> MTIKVGINGFGRIGRIVFRAAQKRSDIEIVAINDLLDADYMAYMLKYDSTHGRFDGTVEVKDGHLIVNGKKIRVTAERDPANLKWDEVGVDVVAEATGLFLTDETARKHITAGAKKVVMTGP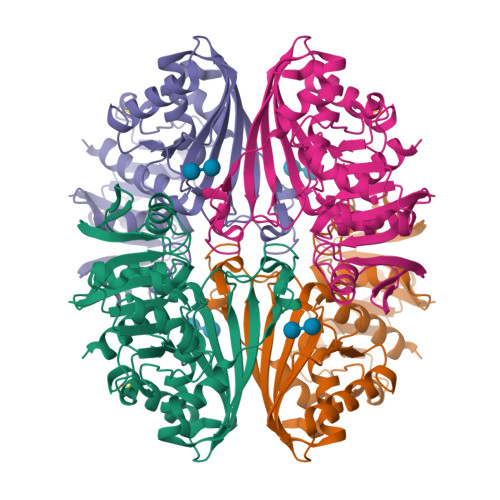SKDNTPMFVKGANFDKYAGQDIVSNASCTTNCLAPLAKVINDNFGIIEGLMTTVHATTATQKTVDGPSHKDWRGGRGASQNIIPSSTGAAKAVGKVLPELNGKLTGMAFRVPTPNVSVVDLTVRLEKAATYEQIKAAVKAAAEGEMKGVLGYTEDDVVSTDFNGEVCTSVFDAKAGIALNDNFVKLVSWYDNETGYSNKVLDLIAHISK> GIKGIYKEIGSGERISLCKLAIDHLEQHNRPLRLAIDMAIWQFQIQAARGGSNPAIRTLFYRFVRLLSLGIHPIFVFDGPNKPIFKRNRRSGTGNGVSTAMAKRLIRLFGFTAHDAPGE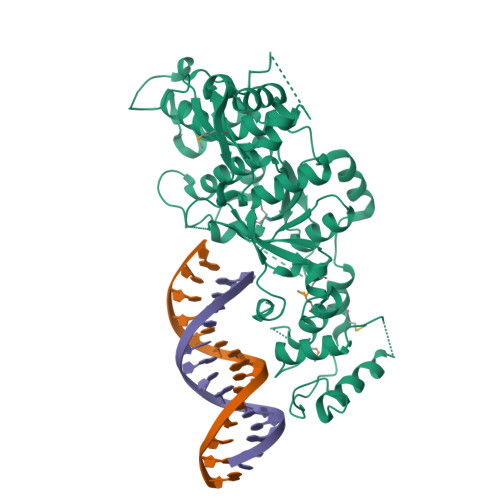AEAECAYLEQQGIVDAVLSEDVDTIMFGSRVTLRDWSSEGSKGGPPTHVTLHDAKKIAEGPSGLDREGMVLVALMSGGDYLPDGIPGCGIKVACQAAKAGFGKELCRIKRADKEAITEWKQRLLHELRTNESGFFRTKHKALEIPENFPNMEVLRYYTHPVVSSPATIERLRQEFPPSSTVDIAGLREFTRETFDWTFRPGAIKLIKVLAPGLLVQRCLDRYVSGPRIDDPDLKKKEESTLVKGISMRREHFSTDATPELRVSFIPAELVGLDPGQEPEVQVEAFGRSGLALNSDDEFDEDISSSQKAPKKPFDPWQPDLAWVPETILKLGVPVTVEDWEEGQRS(2~{R})-2-azanyl-~{N}-[4-ethanoyl-5-(3-hydroxyphenyl)-1,3-thiazol-2-yl]propanamide | C14 H15 N3 O3 S | 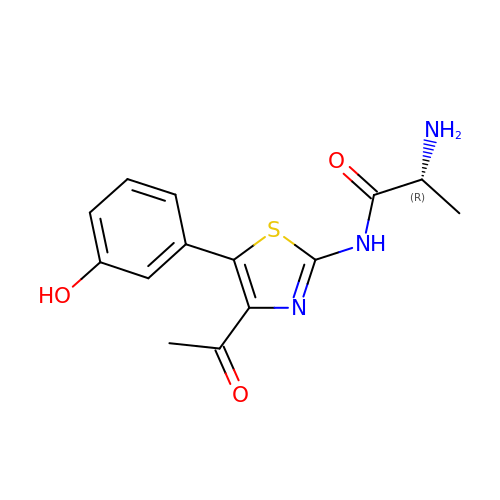GDTJBYZKZGXLNU-SSDOTTSWSA-N> MAFVSGSFGPASALVAQPKRAVSAQRRGVVAMSAAGKKAQQMAALAVAQVAVAMPALAAEGTG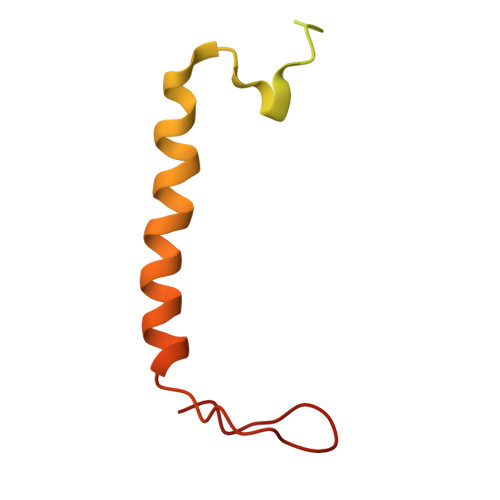AALGVEEPLLFLPLILIPSVFFILFLGFSNKQPKDDFFGAKDDRRN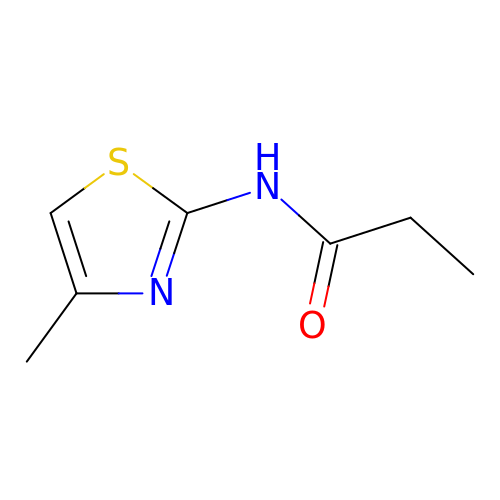N-(4-methyl-1,3-thiazol-2-yl)propanamide | C7 H10 N2 O S | AIOZNYOAFODHNA-UHFFFAOYSA-N> GNCWLRQAKNGRCQVLYKTELSKEECCSTGRLSTSWTEEDVNDNTLFKWMIFNGGAPNCIPCKETCENVDCGPGKKCRMNKKNKPRCVCAPDCSNITWKGPVCGLDGKTYRNECALLKARCKEQPELEVQYQGR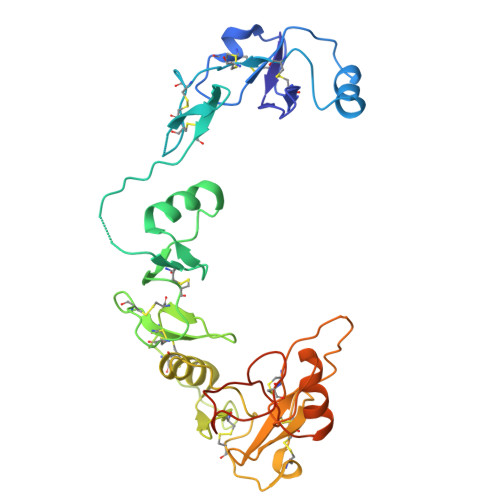CKKTCRDVFCPGSSTCVVDQTNNAYCVTCNRICPEPASSEQYLCGNDGVTYSSACHLRKATCLLGRSIGLAYEGKCIKAKSCEDIQCTGGKKCLWDFKVGRGRCSLCDELCPDSKSDEPVCASDNATYASECAMKEAACSSGVLLEVKHSGSCNSISEDTEEEEEDEDQDYSFPISSILEW> SGLEVLFQGPRSDAERGVCACPRIYMPVCGSNLKTYNNDCLLRCEINSDLGRANNLRKIADQACDNLTDNVNDFIPQEY;> SGLVPRGSSFDCGKPQVEPKKC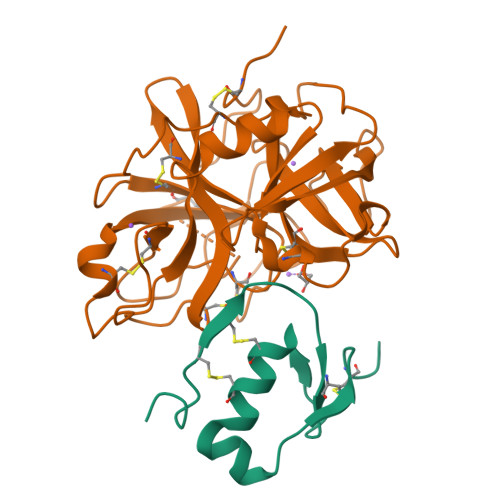PGRVVGGCVAHPHSWPWQVSLRTRFGMHFCGGTLISPEWVLTAAHCLEKSPRPSSYKVILGAHQEVNLEPHVQEIEVSRLFLEPTRKDIALLKLSSPAVITDKVIPACLPSPNYVVADRTECFITGWGETQGTFGAGLLKEAQLPVIENKVCNRYEFLNGRVQSTELCAGHLAGGTDSCQGDSGGPLVCFEKDKYILQGVTSWGLGCARPNKPGVYVRVSRFVTWIEGVMRNN>MGKVYKKVELVGTSEEGLEAAIQAALARARKTLRHL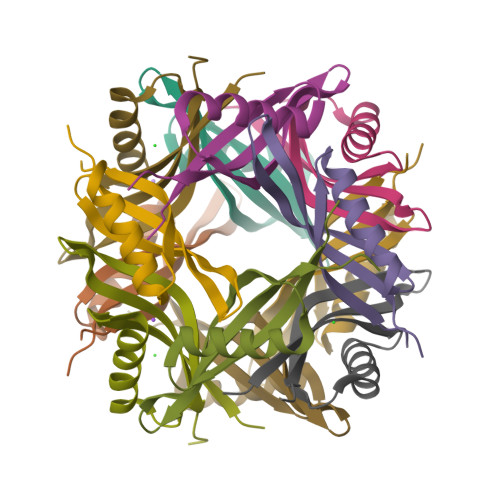DWFEVKEIRGTIGEAGVKEYQVVLEVGFRLEET[6x]> MGRENVLPVHNDVYEDFVFTTPYFQPESTFKSVPKLFSDILLGGVEWVYTTSESVLAYDYKLWYLWSGVSNLDESFDMFFNQYWALSLSTSVFQLFYAVILDRYLSVLFQNTPYTNDWFRMMLHSKETALIWLYHPELSWHINGLNQFFTYFYGGILEFVYFDKSNPDMCILVHTLWIHLLILFLIFTGFVTILFSFYGNPNTEENTIDSDYLAASGTVE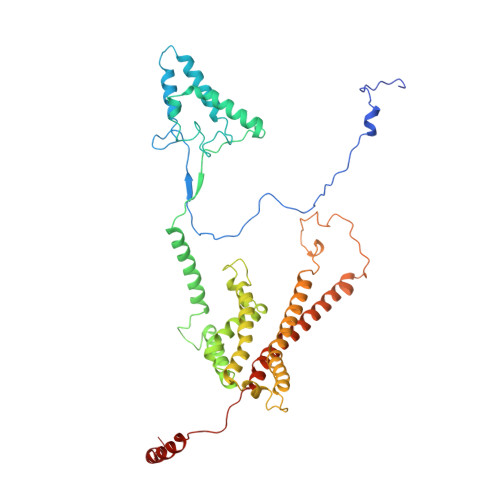AEKEITSIDDYLGLVFAIAYVFGVFFYVHGWTSMLSHAVLLLSCYSIIIMFLFILGMPTLLLYDFGIFFLAYLKGAGKYISSVAEMMFDYTACLVFYIRILAQWIRVVLMVVTFISLSHYVSDFDITNSALIGSENQSDSMNELNTNFSMTYYILTVLPGKFIYWIYEILHTFFVVCSQFVAFFAIVFWLFLFLYTFFIIEKHEDFFSKKREERKKKLKELWNLKN>GSAKDPMTLKEQILNDIKEAMKQKDDFKRDSLRTLNAAFKQIEVDERIELDNERIYKIIASEIKKRKDAIELYLKANREDLAQKEQNEISLFEIYLPKQLSDEELTLALKQLIEELGVSSLKEQGLVMKEAKIKLGASVDGKRLN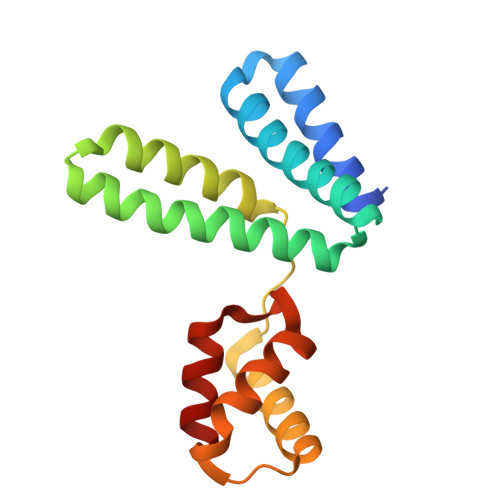LALKELLQ[4x]> PQPCLTGPRTCKDLLDRGHFLSGWHTIYLPDCRPLTVL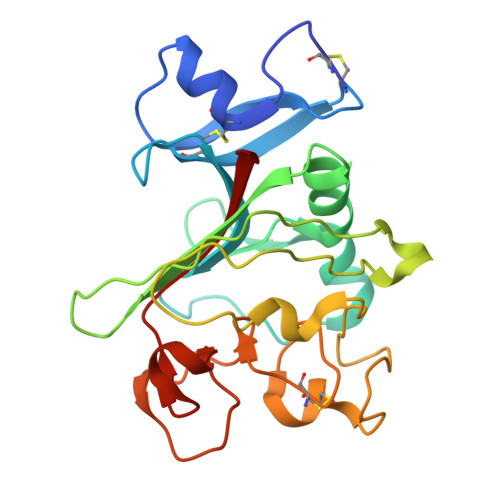CDMDTDGGGWTVFQRRVDGSVDFYRDWATYKQGFGSRLGEFWLGNDNIHALTAQGTSELRTDLVDFEDNYQFAKYRSFKVADEAEKYNLVLGAFVEGSAGDSLTFHNNQSFSTKDQDNDLNNGNCAVMFQGAWWYKNCHTSNLNGRYLRGTHGSFANGINWKSGKGYNYSYKVSEMKVRPA Using IS21 as a model transposase system, we show how an ATPase regulator uses nucleotide-controlled assembly and DNA deformation to enable structure-based site selectivity, transposase recruitment, and activation and integration. The IstA transposase possess two helix-turn-helix (HTH) DNA-binding domains, a DDE catalytic motif and a β-barrel followed by a flexible carboxy-terminal region21. IstB, similar to the MuB and TnsC helper proteins, is a member of the AAA+ family and a close paralogue of the DnaC/I helicase loader. However, this tetramer state is inactive and requires the regulatory IstB factor to perform transposition.

We therefore used an IstB mutant with reduced ATPase and integration activity (Walker B; E167Q) to form a more stable complex that seemed identical to that formed by the wild-type proteins. The cryo-EM structure showed that the IS21 holo-transpososome is formed by one IstA tetramer and two IstB decamers. Two IstB decamers are also seen to dimerize in the presence of the transposase. Notably, they do not assemble into a continuous filament but instead interact in a head-to-head configuration (that is, through the interior terminal dimers of each decamer, labelled 1 and 1′ in Fig. 2c). However, the interaction between the two IstB decamers also induces the DNA to adopt a sharp deformation at their junction to give rise to a kinked S-shaped configuration overall. In particular, the dyad-proximal AAA+ subunits of IstB, for which nucleotide-binding sites are oriented towards IstA (monomers 1a and 1a′), interact with the catalytic monomers of the transposase. For IstA, this recognition occurs through the C-terminal β-barrels of the catalytic transposase subunits that are flexibly tethered to the DDE domains of the enzyme. These elements dock into a deep exterior cleft formed between the N-terminal dimerization and C-terminal ATPase domains of IstB. We therefore performed both particle subtraction (to remove the flexible parts of the transposase and the AAA+ oligomers) and focused refinement of the holo-transpososome core; the resultant 3.2 Å reconstruction of IstA-bound IstB revealed that the density in these active sites is most consistent with ADP. In particular, new and specific contacts established between the β-barrels and the DDE modules of the lower-most (integration-site proximal) IstA monomers with the IstB ATPase induce a large-scale rotation of the integrase domains (72°). This conformational change helps to reorientate the catalytic triad of the transposase into the appropriate spacing and geometry to perform transposition.

>[4x]MITRGEFFMIKEMYERGMSISDIARELGIDRKTVRKYIHSPNPPSKSKRKQRKSKLDPFKPYLQKRMLEDGVFNSEKLFFEIRQQGYTGGKTILKDYMKPFRETAKKKYTVRYETLPGEQMQVDWKEVGEVVIEGKKVKLSLFVATLGYSRMKYAVFTTSQDQEHLMECLIQSFKYFGGVPKKVLFDNMKTVTDGREQGVVKWNQRFSEFASYYGFIPKVCRPYRAQTKGKVERAIQYIMDHFYVGTAFESIEELNFLLHRWLDQVANRKPNATTGISPQERWAEESLKPLPLKDYDTSYLSYRKVHWDGSFSYKGEQWLLSAEYAGKEILVKERLNGDIRLYFRGEEISHVDQQKKVISFAEKIKKKQTEMA;>NMKERIHEYCHRLHLPVMAERWSAMAEYASTHNISYSEFLFRLLEAEIVEKQARSIQTLIKLSKLPYRKTIDTFDFTAQPSVDERRIRELLTLSFIDRKENILFLGPPGIGKTHLAISIGMEAIARGYKTYFITAHDLVNQLRRADQEGKLEKKLRVFVKPTVLIIDQMGYLKLDPNSAHYLFQVIARRYEHAPIILTSNKSFGEWGEIVGDSVLATAMLDRLLHHSIIFNLKGESYRLREKRLQEE[20x]> PTPCYISIEGQTQGLITAGACTADSIGDSFVEGHEDEMLVQQFDHVVTVPTDPQSGQPSGQRVHK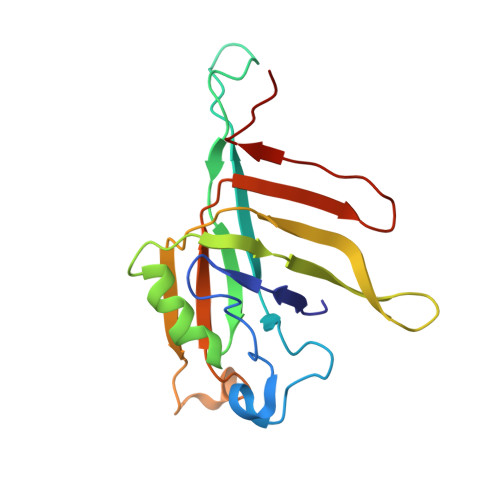PFKFTVALNKAVPLLYNALSSGEKLKTVELKWYRTSIEGKQENFFTTKLENASIVDIHCEMPHCQDPAKSDFTQNVTVSLSYRKITWDHVNAGTSGSDDWRKPIE>[2x]MAHHHHHHMSKVTLGGNPIDLAGTFPAVG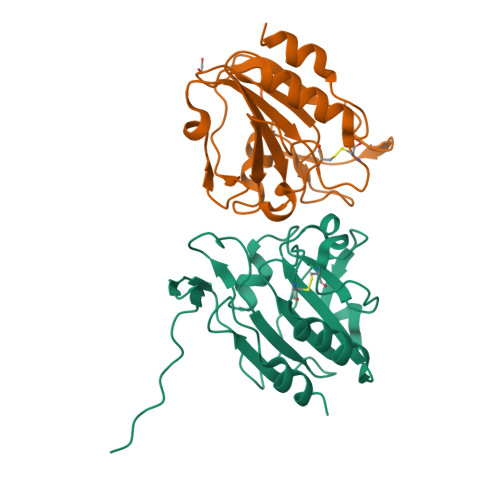AQAADFKLVGKDLADLSLASFAGKRKVLNIVPSLDTPTCATSTRKFNEAASSLDNTVVIVVSADLPFAATRFCTTEGLANVVTASTFRTGRAFANAYGVDVTSGPLNGLTARAVVVLDAQDKVIHAELVGEIKDEPNYDAALAALK Voltage-gated sodium (Nav) channels govern membrane excitability in neurons and muscles. Nav1.7, encoded by SCN9A and primarily localized to the dorsal root ganglion neurons, has been explored as a prominent target for pain management. The S1-S4 segments in each repeat constitute the flanking voltage-sensing domain (VSD), and the S5-S6 segments enclose the PD that is responsible for selective and gated ion permeation. Here we report high-resolution cryo-EM structures of human Nav1.7 treated with drugs and lead compounds with representative chemical backbones at resolutions of 2.6-3.2 Å.

Our incentive to solve the structure of PF-05089771 bound to wild-type (WT) human Nav1.7 was to verify if the chimeric VSD can faithfully recapitulate all binding details. The binding mode of PF-05089771 in the intact Nav1.7-VSDIV is remarkably similar to the chimeric one. As coordination details and the molecular basis for the subtype-specificity have been thoroughly discussed by Ahuja and co-workers, we will not elaborate on this one. Whereas small molecules like PF-05089771 resides in an extracellular cavity of VSDIV, peptide toxins like ProTx-II and HWTX-IV bind to the extracellular periphery of the VSD, partly immersed in the lipid bilayer. Per this definition, PF-05089771 binds to site V4EC, HWTX-IV and LqhIII to V4EM, and Dc1a to site V2EP. Site V4C has been extensively explored for subtype-specific antagonists, such as PF-05089771 for Nav1.7 and ICA121431 for Nav1.3.

> MAMLPPPGPQSFVHFTKQSLALIEQRIAERKSKEPKEEKKDDDEEAPKPSSDLEAGKQLPFIYGDIPPGMVSEPLEDLDPYYADKKTFIVLNKGKTIFRFNATPALYMLSPFSPLRRISIKILVHSLFSMLIMCTILTNCIFMTMNNPPDWTKNVEYTFTGIYTFESLVKILARGFCVGEFTFLRDPWNWLDFVVIVFAYLTEFVNLGNVSALRTFRVLRALKTISVIPGLKTIVGALIQSVKKLSDVMILTVFCLSVFALIGLQLFMGNLKHKCFRNSLENNETLESIMNTLESEEDFRKYFYYLEGSKDALLCGFSTDSGQCPEGYTCVKIGRNPDYGYTSFDTFSWAFLALFRLMTQDYWENLYQQTLRAAGKTYMIFFVVVIFLGSFYLINLILAVVAMAYEEQNQANIEEAKQKELEFQQMLDRLKKEQEEAEAIAAAAAEYTSIRRSRIMGLSESSSETSKLSSKSAKERRNRRKKKNQKKLSSGEEKGDAEKLSKSESEDSIRRKSFHLGVEGHRRAHEKRLSTPNQSPLSIRGSLFSARRSSRTSLFSFKGRGRDIGSETEFADDEHSIFGDNESRRGSLFVPHRPQERRSSNISQASRSPPMLPVNGKMHSAVDCNGVVSLVDGRSALMLPNGQLLPEVIIDKATSDDSGTTNQIHKKRRCSSYLLSEDMLNDPNLRQRAMSRASILTNTVEELEESRQKCPPWWYRFAHKFLIWNCSPYWIKFKKCIYFIVMDPFVDLAITICIVLNTLFMAMEHHPMTEEFKNVLAIGNLVFTGIFAAEMVLKLIAMDPYEYFQVGWNIFDSLIVTLSLVELFLADVEGLSVLRSFRLLRVFKLAKSWPTLNMLIKIIGNSVGALGNLTLVLAIIVFIFAVVGMQLFGKSYKECVCKINDDCTLPRWHMNDFFHSFLIVFRVLCGEWIETMWDCMEVAGQAMCLIVYMMVMVIGNLVVLNLFLALLLSSFSSDNLTAIEEDPDANNLQIAVTRIKKGINYVKQTLREFILKAFSKKPKISREIRQAEDLNTKKENYISNHTLAEMSKGHNFLKEKDKISGFGSSVDKHLMEDSDGQSFIHNPSLTVTVPIAPGESDLENMNAEELSSDSDSEYSKVRLNRSSSSECSTVDNPLPGEGEEAEAEPMNSDEPEACFTDGCVWRFSCCQVNIESGKGKIWWNIRKTCYKIVEHSWFESFIVLMILLSSGALAFEDIYIERKKTIKIILEYADKIFTYIFILEMLLKWIAYGYKTYFTNAWCWLDFLIVDVSLVTLVANTLGYSDLGPIKSLRTLRALRPLRALSRFEGMRVVVNALIGAIPSIMNVLLVCLIFWLIFSIMGVNLFAGKFYECINTTDGSRFPASQVPNRSECFALMNVSQNVRWKNLKVNFDNVGLGYLSLLQVATFKGWTIIMYAAVDSVNVDKQPKYEYSLYMYIYFVVFIIFGSFFTLNLFIGVIIDNFNQQKKKLGGQDIFMTEEQKKYYNAMKKLGSKKPQKPIPRPGNKIQGCIFDLVTNQAFDISIMVLICLNMVTMMVEKEGQSQHMTEVLYWINVVFIILFTGECVLKLISLRHYYFTVGWNIFDFVVVIISIVGMFLADLIETYFVSPTLFRVIRLARIGRILRLVKGAKGIRTLLFALMMSLPALFNIGLLLFLVMFIYAIFGMSNFAYVKKEDGINDMFNFETFGNSMICLFQITTSAGWDGLLAPILNSKPPDCDPKKVHPGSSVEGDCGNPSVGIFYFVSYIIISFLVVVNMYIAVILENFSVATEESTEPLSEDDFEMFYEVWEKFDPDATQFIEFSKLSDFAAALDPPLLIAKPNKVQLIAMDLPMVSGDRIHCLDILFAFTKRVLGESGEMDSLRSQMEERFMSANPSKVSYEPITTTLKRKQEDVSATVIQRAYRRYRLRQNVKNISSIYIKDGDRDDDLLNKKDMAFDNVNENSSPEKTDATSSTTSPPSYDSVTKPDKEKYEQDRTEKEDKGKDSKESKK;> MGRLLALVVGAALVSSACGGCVEVDSETEAVYGMTFKILCISCKRRSETNAETFTEWTFRQKGTEEFVKILRYENEVLQLEEDERFEGRVVWNGSRGTKDLQDLSIFITNVTYNHSGDYECHVYRLLFFENYEHNTSVVKKIHIEVVDKANRDMASIVSEIMMYVLIVVLTIWLVAEMIYCYKKIAAATETA;> MHRDAWLPRPAFSLTGLSLFFSLVPPGRSMEVTVPATLNVLNGSDARLPCTFNSCYTVNHKQFSLNWTYQECNNCSEEMFLQFRMKIINLKLERFQDRVEFSGNPSKYDVSVMLRNVQPEDEGIYNCYIMNPPDRHRGHGKIHLQVLMEEPPERDSTVAVIVGASVGGFLAVVILVLMVVKCVRRKKEQKLSTDDLKTEEEGKTDGEGNPDDGAK>AATDISGAFEYSGWENFHRTQWSWDKKTRGAHLVNCTGACPHFVYSKDGVVMREEQSKDIAPMPNIPEYNPRGCNKGECGHDYMYGPHRIKYPLIRVGERGEGKWRRATWEEALDMIADKCVDTIKNHAPDCISVYSPVPAVSPVSFSAGHRFAHYIGAHAHTFYDWYGDHPTGQTQTCGVQGDTCETADWFNSKYIILWGSNPTQTRIPDAHFLSEAQLNGAKIVSISPDYNSSTIKVDKWIHPQPGTDGALAMAMAHVIIKEKLYDAHSLKEQTDLSYLVRSDTKRFLREADVVAGGSKDKFYFWNAKTGKPVIPKGSWGDQPEKKGSPVGFLGRNTFAFPKGYIDLGDLDPALEGKFNMQLLDGKTVEVRPVFEILKSRLMADNTPEKAAKITGVTAKAITELAREFATAKPSMIICGGGTQHWYYSDVLLRAMHLLTALTGTEGTNGGGMNHYIGQEKPAFVAGLVALAFPEGVNKQRFCQTTIWTYIHAEVNDEIISSDIDTEKYLRDSITTGQMPNMPEQGRDPKVFFVYRGNWLNQAKGQKYVLENLWPKLELIVDINIRMDSTALYSDVVLPSAHWYEKLDLNVTSEHSYINMTEPAIKPMWESKTDWQIFLALAKRVEMAAKRKKYEKFNDEKFKWVRDLSNLWNQMTMDGKLAEDEAAAQYILDNAPQSKGITIQMLREKPQRFKSNWTSPLKEGVPYTPFQYFVVDKKPWPTLTGRQQFYLDHDTFFDMGVELPTYKAPIDADKY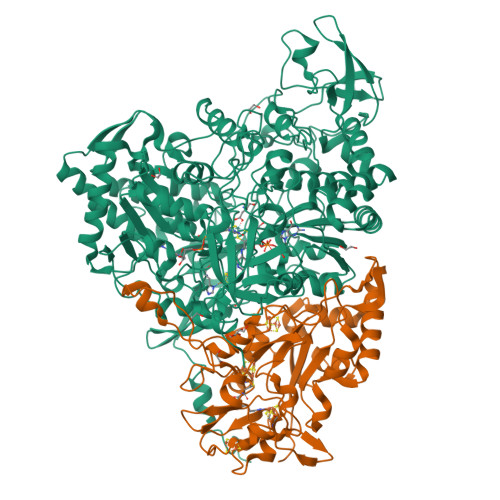PFRFNSPHSRHSVHSTFKDNVLMLRLQRGGPSIEMSPLDAKPLGIKDNDWVEAWNNHGKVICRVKIRNGEQRGRVSMWHCPELYMDLLTGGSQSVCPVRINPTNLVGNYGHLFFRPNYYGPAGSQRDVRVNVKRYIGATPISF[6x];>MANVMKAPRRQLTYVTDLNKCIGCQTCTVACKKLWTTGPGQDFMYWRNVETAPGLGYPRNWQTKGGGYKNGELQKGKIPPMIDYGIPFEFDYAGRLFEGKPGRVRPSPTPRSAPNWDEDQGAGEYPNNSFFYLPRMCNHCTKPACLEACPNEAIYKREQDGIVVIHQDKCKGAQACVQSCPYAKPYFNPLTNKANKCIGCFPRIEQGVAPACVAQCVGRAMHVGFVDDVNSSVYKLIKQYKVALPLHPEFGTEPNVFYVPPVLGPRIEMANGEPSTDPKIPLAQLEGLFGKQVRDVLAILQSEREKKMKGLASDLMDVLIGRRSTDMMISPLT[6x]> SMNKLYIGNLSDHAGPADLESVFKDAKIPVAGPFLVKTGYAFVDCPDEGWALKAIEALSGKMELHGKPMEVEHSVPKRQRIRKLQIRNIPPHLQWEVLDSLLVQYGVVESCEQVNTDSETAVVNVTYSSKDQA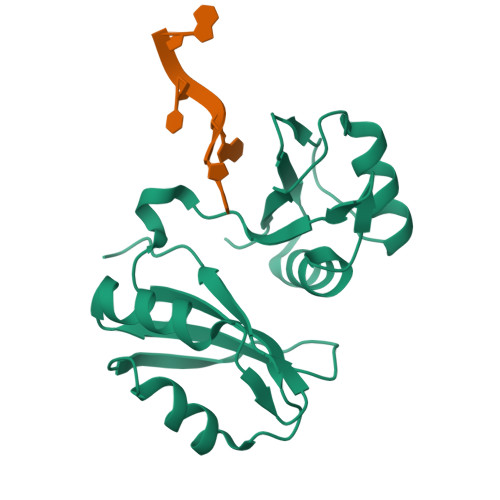RQALDKLNGFQLENFTLKVAYIPDETAAA As a proof-of-concept, five peptidoglycan hydrolases from the Acinetobacter baumannii proteome (PHAb7-PHAb11) were identified using PlyF307 lysin-derived peptide as a template. To understand the catalytic mechanism and thermal stability of these peptidoglycan hydrolases, we attempted to decipher their structures and eventually obtained the crystal structures of PHAb8, PHAb10, and PHAb11 by X-ray crystallography. Despite their lower amino acid sequence similarity, PHAb8, PHAb10, and PHAb11 superimposed well with T4 lysozyme, especially in their Glu-Asp-Thr catalytic triad regions, suggesting that PHAb8, PHAb10, and PHAb11 may be phage-originated. All these observations together indicated that PHAb8, PHAb10, and PHAb11 were highly evolutionarily related to T4 lysozyme and might share similar catalytic mechanisms of action.

Results showed that PHAb8 was a monomer, while PHAb10 and PHAb11 formed an asymmetric dimer. Specifically, the two asymmetric units of PHAb10 formed an antiparallel dimer with a rotation angle of 177.2° along the rotation axis and a distance of 10.5 Å between them. Further, PHAb10 dimer adopted a circularly permuted architecture, in which the N-terminus of one chain and the C-terminus of another chain formed a cavity, which might be the binding site of the peptidoglycan substrate. Structure-based homology analysis revealed that PHAb10 and PHAb11 probably belonged to the T4 lysozyme family and possessed the conserved Glu-Asp-Thr catalytic triad shared by traditional phage lysins and bacterial autolysins, namely Glu17, Asp26, and Thr32 of PHAb10, and Glu52, Asp61, and Thr67 of PHAb11. We carefully examined the topology of the PHAb10 dimer and found that it was supported by seven pairs of intermolecular H-bonds, with three pairs supporting the head, each two pairs in midbody and tail of the PHAb10 dimer. Specifically, in the top view of chain A, Arg20 and Gly27 were involved in intermolecular H-bond interactions, supporting the head region, Gly128 and Gly129-mediated interaction contributed to the stability of midbody, while Lys133 and Arg137 were involved in intermolecular H-bond forces anchoring the tails of the PHAb10 dimer. While the variants R20IG27D, which has mutations in the head-supporting site, and G27DR137I, which has mutations in both the head and tail supporting sites, lost dimerization ability. As a result, both variants lost most of their bactericidal activity after treatment at 100°C for 1 hr, which could be further explained by the failure to recover their native forms after heat treatment. At temperatures above its transition point (i.e. >53.7°C), dimerized PHAb10 dissociated into monomers without precipitation. During the cooling process, monomeric PHAb10 refolded to a stable dimer via the intermolecular interactions between the two monomers, i.e., three pairs of intermolecular bonds at the head, two in the midbody, and two at the tail of the PHAb10 dimer.

>MSKTTSNAGLNLIKGFEGKRLNAYDDGVGVWTIGFGTIKYPNGVRVKKGDTCTEQQAETYLKNDLTKFEVAINKLVKVSLTQNQFDALASFTYNLGETNLANSTLLKKLNKGDYQGAADQFLVWNKAGGKVMKGLVRRREAERALFLKK[2x]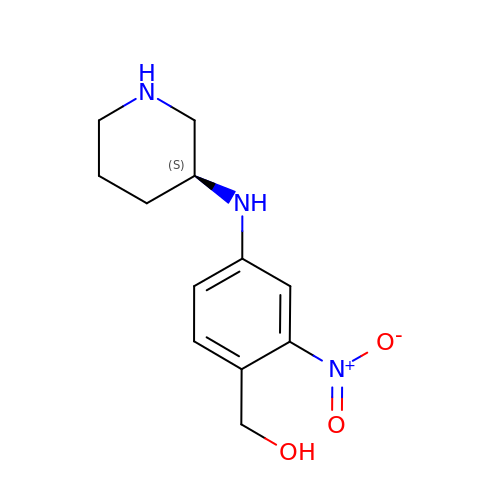(2-nitro-4-{[(3S)-piperidin-3-yl]amino}phenyl)methanol | C12 H17 N3 O3 | UMHUFFXXYSYMND-NSHDSACASA-N> DNQFYSVEVGDSTFTVLKRYQNLKPIGSGAQGIVCAAYDAVLDRNVAIKKLSRPFQNQTHAKRAYRELVLM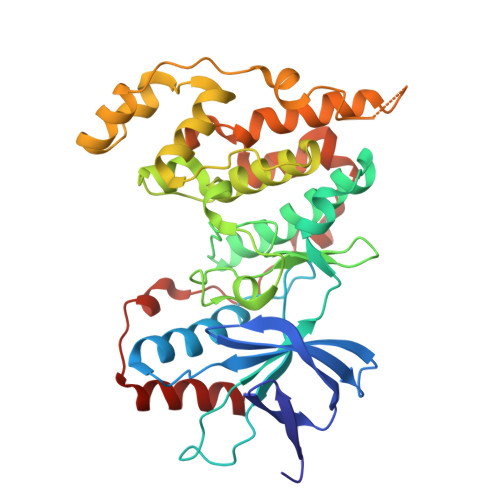KCVNHKNIISLLNVFTPQKTLEEFQDVYLVMELMDANLCQVIQMELDHERMSYLLYQMLCGIKHLHSAGIIHRDLKPSNIVVKSDCTLKILDFGLARTAGTSFMMTPYVVTRYYRAPEVILGMGYKENVDIWSVGCIMGEMVRHKILFPGRDYIDQWNKVIEQLGTPCPEFMKKLQPTVRNYVENRPKYAGLTFPKLFPDSLFPADSEHNKLKASQARDLLSKMLVIDPAKRISVDDALQHPYINVWYDPAEVEAPPPQIYDKQLDEREHTIEEWKELIYKEVMN[9-[2-carboxy-5-[2-[2-[5-(methylsulfonylamino)pentoxy]ethoxy]ethylcarbamoyl]phenyl]-6-(dimethylamino)xanthen-3-ylidene]-dimethyl-azanium | C35 H45 N4 O8 S | 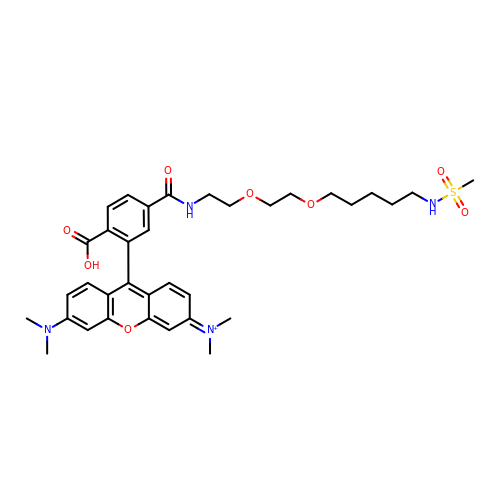AKUULRQTVFOLNZ-UHFFFAOYSA-O> GNKICQFKLVLLGESEVGKSSLVLRFVKGQFHEFQESTIGA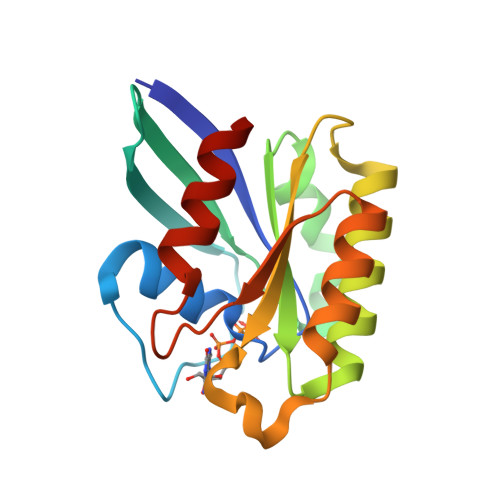AFLTQTVCLDDTTVKFEIWDTAGQERYHSLAPMYYRGAQAAIVVYDITNEESFARAKNWVKELQRQASPNIVIALSGNKADLANKRAVDFQEAQSYADDNSLLFMETSAKTSMNVNEIFMAIAKKLPKN methyl 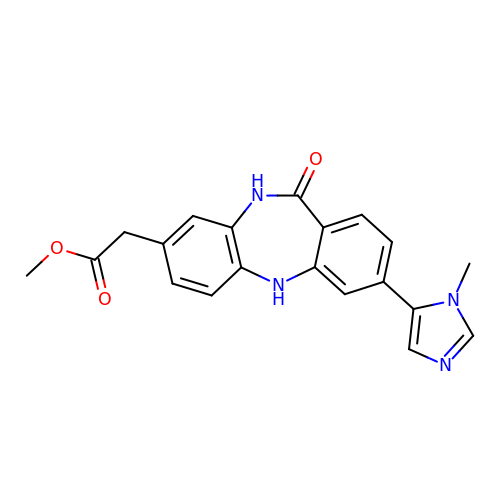[3-(1-methyl-1H-imidazol-5-yl)-11-oxo-10,11-dihydro-5H-dibenzo[b,e][1,4]diazepin-8-yl]acetate | C20 H18 N4 O3 | VHPMIVHLGSAOKI-UHFFFAOYSA-N> GSMALEQALQAARRGDLDVLRSLHAAGLLGPSLRDSLDALPVHHAARSGKLHCLRYLVEEVALPAVSRARNGATPAHDAAATGYLSCLQWLLTQGGCRVQEKDNSGATVLHLAARFGHPDVVKWLLYQGGANSAITTDTGALPIHYAAAKGDLPSLKLLVGHYPEGVNAQTNNGATPLYLACQEGHLEVTKYLVQECSADPHLRAQDGMTPLHAAAQMGHNPVLVWLVSFADVSFSEQDHDGATAMHFAASRGHTKVLSWLLLHGAEISQDLWGGTPLHD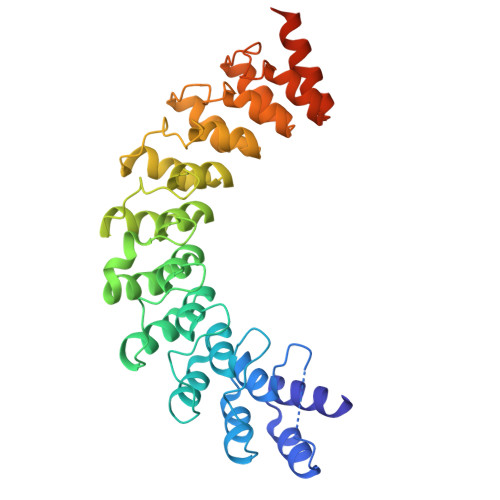AAENGELECCQILAVNGAGLDVRDHDGYTAADLAEFNGHTHCSRYLRTVQTLSLEHRVLSRDQSMDLEAKQLDS> MKRKLFWICAVAMGMSAFPSFMTQATPATQPLINAEPAVAAQTEQNPQVGQVMPGVQGADAPVVAQNGPSRDVKLTFAQIAPPPGSMVLRGINPNGSIEFGMRSDEVVTKAMLNLEYTPSPSLLPVQSQLKVYLNDELMGVLPVTKEQLGKKTLAQMPINPLFISDFNRVRLEFVGHYQDVCEKPASTTLWLDVGRSSGLDLTYQTLNVKNDLSHFPVPFFDPSDNRTNTLPMVFAGAPDVGLQQASAIVASWFGSRSGWRGQNFPVLYNQLPDRNAIVFATNDKRPDFLRDHPAVKAPVIEMINHPQNPYVKLLVVFGRDDKDLLQAAKGIAQGNILFRGESVVVNEVKPLLPRKPYDAPNWVRTDRPVTFGELKTYEEQLQSSGLEP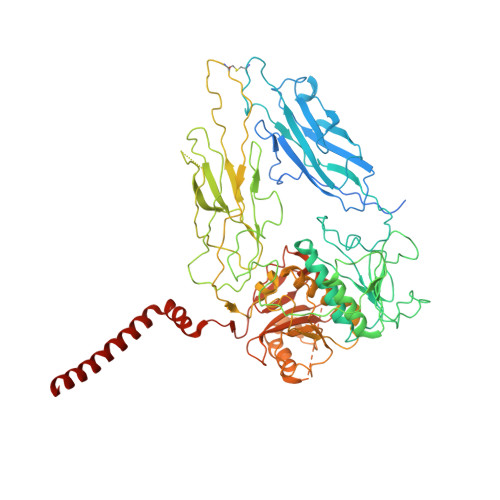AAINVSLNLPPDLYLMRSTGIDMDINYRYTMPPVKDSSRMDISLNNQFLQSFNLSSKQEANRLLLRIPVLQGLLDGKTDVSIPALKLGATNQLRFDFEYMNPMPGGSVDNCITFQPVQNHVVIGDDSTIDFSKYYHFIPMPDLRAFANAGFPFSRMADLSQTITVMPKAPNEAQMETLLNTVGFIGAQTGFPAINLTVTDDGSTIQGKDADIMIIGGIPDKLKDDKQIDLLVQATESWVKTPMRQTPFPGIVPDESDRAAETRSTLTSSGAMAAVIGFQSPYNDQRSVIALLADSPRGYEMLNDAVNDSGKRATMFGSVAVIRESGINSLRVGDVYYVGHLPWFERVWYALANHPILLAVLAAISVILLAWVLWRLLRIISRRRLNPDNE>[4x]MPPVSSARNLKELPKFRDGLSYLYVEHAVVEREAGGIGIYDQEGLTLAPVA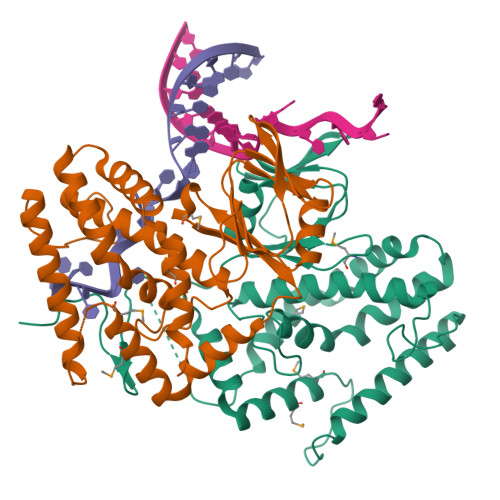GLGVLFLGPGTRITHAAVRLLAENGCTVAWVGEGMARFYAQGLGDTRSAARFYRQARAWADPALHLEVVMRLYRMRFSEPLPEGLTLEQVRGLEGVRVRNAYARWSRETGVPWYGRSYDRGNWRAADPVNRALSAGASYLYGLAHAAIVSLGFSPALGFIHTGKLLSFVYDIADLYKADYLVPAAFRTVAESEEAVERRVRRALREAIQEGRLLERMAEDLLNLFRGLGLPEEEDPVEEDPTRPGGLWDLEGEVEGGVAYGGDDPGEGAEEPEG>[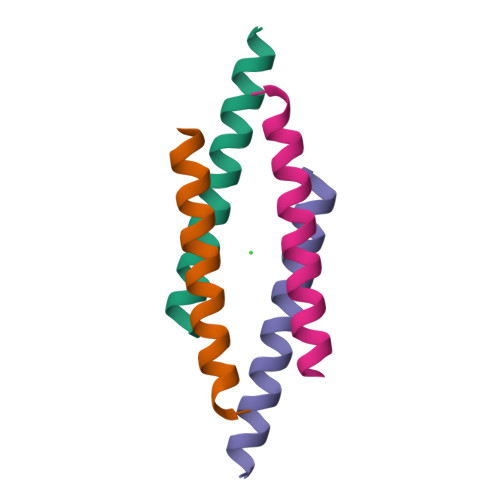2x]LLGDFFRKSKEKIGKEFKRIVQRIKDFLRNLVPRTES Here, we report the biochemical and structural characterization of two membrane-bound MBLs: CJO-1 and CIM-2, from Chryseobacterium joostei and Chryseobacterium indologenes, respectively. Both MBLs confer β-lactam resistance on producer bacterial strains and hydrolyze several antibiotics, although with impaired efficiency compared to NDM-1. The structures confirmed that both proteins adopt the characteristic αβ/βα sandwich fold of B1 subclass MBL enzymes (0.59 Å root mean square deviation [RMSD], over 220 Cα of CJO-1 with CIM-2), with two Zn(II) ions in their active sites (respectively). Specifically, a hindered access to the active site with the contribution of a Tyr residue in loop L10 and the presence of a positively charged Lys residue in loop L3 limit hydrolysis of cephalosporins with charged C3 substituents.

Aiming to understand the substrate profile of these enzymes, we crystallized both CJO-1 and CIM-2 in their soluble forms and solved their X-ray structures using single wavelength anomalous dispersion (SAD) from data collected at the Zn edge. CIM-2 diffraction data extended to 1.56 Å resolution, and CJO-1 to 1.34 Å. CJO-1 could be modeled with a partially oxidized Cys221, as has been observed previously in crystal structures of the B1 MBL VIM-2 (33), with 13% occupancy for a sulfenic acid. In the simulations of CJO-1, both loops remain closer to the active site, resulting in hindered access for β-lactams with bulky substituents, like piperacillin, which showed the lowest catalytic efficiency among the tested β-lactams. Among these substitutions, the presence of a lysine at position 59 (with a positively charged side chain) also modifies the surface charge distribution of CJO-1 when compared to NDM-1. This surface charge distribution is likely to generate repulsive interactions with substrates with a positive charge density in their substituents, as in the bicyclic β-lactams tested with positive charges in their C2/C3 substituents, e.g., cefepime, ceftazidime, or imipenem. Overall, the combined effects of Leu59Lys and Asn233Tyr substitutions in CJO-1 introduce a steric-electrostatic effect on the surface of the protein surrounding the active site. We generated the Lys59Leu variant of CJO-1, and we determined the resistance phenotype of E. coli cells expressing this variant. This replacement increased the MIC of cefepime, the poorest substrate of CJO-1, by almost one order of magnitude, with reduced impact on the MIC values of cefotaxime and ceftazidime. Despite other features that can fine-tune the reactivity, we conclude that the main determinant of the distinct substrate profile of CJO-1 against cefepime is based on the electrostatic repulsion with the positive charge of the lys59 residue.

> GHMSSQHAEKFRAKEIYKSENLIITQISENSFIHTSFKQTNDFGNVPCNGLIVKNNDETIVFDTPTNDKDSEELIQWITGTLHSKINAVIPTHFHDDSMGGLQAFHNHNIPSYSYSKTIELGKENNFVVPKNSFNNFITLKVGNEEVIAKFFGEGHTRDNTVGYFPSENILFGGCLLKELEASKGYLGDANVSAWSSTVEKVKKEYPNVKIVIPGHGEYGDKKLLDYTIKLFKTP>[4x]MAEAGITGTWYNQLGSTFIVTAGADGALTGTYESAVGNAESRYVLTGRYDSAPATDGSGTALGWTVAWKNNYRNAHSATTWSGQYVGGAEARINTQWLLTSGTTEANAWKSTLVGHDTFTKVKPSAAS

Tetrameric streptavidin (T-Sav) has been popularly used, engineered and evolved for hosting reactions that are mediated by biotin-appended chemical catalysts. We have recently reported an organocatalytic 1,4 conjugate addition of nitromethane to cinnamaldehydes within a protein environment through adaptation of the streptavidin–biotin technology. In this system, biotin was covalently modified with pyrrolidine groups, resulting in ligands 1 and 2 which differ by one stereocenter. Here, we performed mechanistic investigations on how a protein host affects iminium catalysis.

In each T-Sav, there are four biotin-binding sites whose arrangement locates the catalyzed reactions at the interface of two subunits which has a C2 symmetry. In previous and current crystallographic studies, Ser112 was found to be in a hydrogen-bonding distance with the reacting nitrogen atom of the pyrrolidine motif. Altogether, this suggests that Ser112 helps in positioning the intermediate for nucleophilic addition at the Cβ position, improving both the regio- and enantioselectivities of the reaction. In contrast, the conversion and stereoselectivity were mildly improved when the T-rSav-L124W variant was used as a host, indicating the importance of placing a bulky and hydrophobic residue at this position (entry 23). The Lys121 residues in both T-Sav subunits (namely SavA and SavB, see below) are also in close proximity to the reacting centers. In contrast, substituting Lys121 with methionine or arginine does not affect the performance of the reaction, implying that the size of the sidechain, rather than its electrostatic properties, is responsible for the observed selectivity (entries 25 and 26). Notably, the Lys121 variants resulted in low 1,2-byproduct formation, indicating that this residue does not improve the regioselectivity of the reaction but plays a role in guiding how the nucleophile (deprotonated nitromethane) approaches the C-4 of the iminium intermediate. The non-linear increase in yield implied that each T-Sav binding site cannot mediate iminium catalysis simultaneously and the intersubunit interface can only host one chemical transformation event at a time. Our mutational, crystallographic and mechanistic studies have indicated that the protein environment corresponding to the subunit interface of T-Sav is critical for catalysis by biotinylated secondary amines. This microenvironment controls the reaction conversion, regioselectivity (1,4- over 1,2-addition) and stereoselectivity (S vs. R).CHLORATE ION | Cl O3 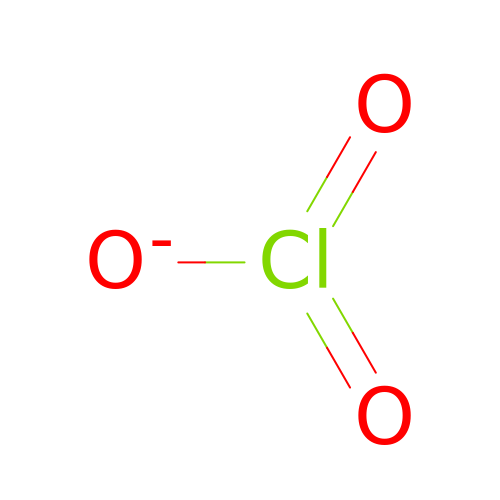| XTEGARKTQYYJKE-UHFFFAOYSA-M> MASPIESARIGEVKRETKQTNVSVKINLDGHGVSDSSTGIPFLDHMLDQLASHGLFDVHVRATGDTHIDDHHTNEDVALAIGTALLKALGERKGINRFGDFTAPLDEALIHVSLDLSGRPYLGYNLEIPTQRVGTYDTQLVEHFFQSLVNTSGMTLHIRQLAGKNSHHIIEATFKAFARALRQATESDPRRGGTIPSSKGVLSRS

Imidazoleglycerol-phosphate dehydratase (IGPD) catalyzes the Mn(II)-dependent dehydration of imidazoleglycerol phosphate (IGP) to 3-(1H-imidazol-4-yl)-2-oxopropyl dihydrogen phosphate during biosynthesis of histidine. The metalloenzyme imidazoleglycerol-phosphate dehydratase (IGPD) (EC 4.2.1.19) has been identified as a potential herbicide target due to its essential role in histidine biosynthesis (Ames, 1957; Hilton et al., 1965). Since the substrate lacks a carbonyl or imine adjacent to the leaving proton, which is thus non-acidic, IGPD uses an unusual mechanism for catalysis that is distinct from other dehydration reactions that have been reported to date (Glynn et al., 2005).

To study substrate binding in IGPD, we used site-directed mutagenesis to produce an inactive mutant of A. thaliana IGPD2 by replacing E21, a putative acid-base catalyst, with a glutamine residue. E21Q IGPD2 was co-crystallized with substrate to yield a 1.12 Å resolution structure of the enzyme-substrate complex, termed form A. In contrast to Mn1, the second manganese ion, Mn2, is five-coordinate, sharing the same four protein ligands (E77, H145, H73, and H170) and one water ligand (HOH1) with those seen in the holoenzyme structure. However, the position of the imidazole-N3 nitrogen atom of the substrate is such that it would be too close to that of HOH2, the sixth Mn2 ligand in the holoenzyme. This potential steric clash in the form A complex is avoided by the prior displacement of HOH2 from the enzyme. The substrate imidazole-N3 nitrogen atom forms a hydrogen bond to HOH1, which in turn is hydrogen bonded to two conserved carboxyl groups (E77 and D108). This arrangement implies that the imidazole ring is neutral, with its N3 nitrogen atom protonated and acting as a hydrogen bond donor, consistent with its high pKa (∼14.5) for deprotonation. The structure of form A therefore shows that IGPD links the binding of its substrate to the generation of a ligand-depleted, five-coordinate Mn(II) ion at the heart of the active site. The form A complex demonstrates how the open form of the enzyme can capture the neutral imidazole form of IGP.>[2x]FADRMVIKAQSPAGFAEEYIIESIWNNRFPPGTILPAERELSELIGVTRTTLREVLQRLARDGW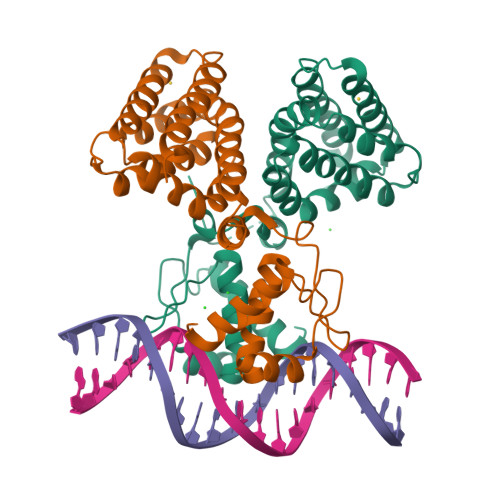LTIQHGKPTKVNNFWETSGLNILETLARLDHESVPQLIDNLLSVRTNISTIFIRTAFRQHPDKAQEVLATANEVADHADAFAELDYNIFRGLAFASGNPIYGLILNGMKGLYTRIGRHYFANPEARSLALGFYHKLSALCSEGAHDQVYETVRRYGHESGEIWHRMQKNLPGDLAIQGR>[4x]SNAMAKLRVGIVFGGKSAEHEVSLQSAKNIVDAIDKTRFDVVLLGIDKAGQWHVNDAENYLQNADDPAHIALRPSAISLAQVPGKHQHQLINAQNGQPLPTVDVIFPIVHGTLGEDGSLQGMLRVANLPFVGSDVLSSAACMDKDV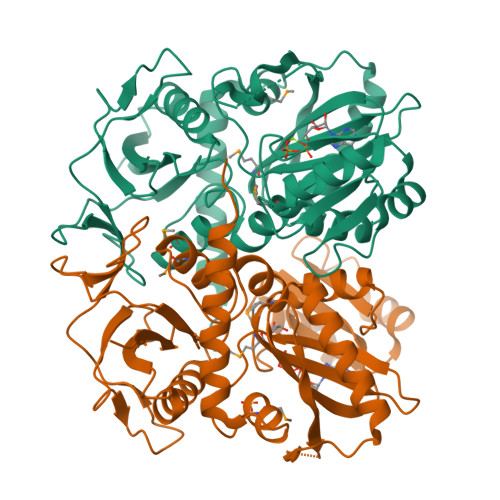AKRLLRDAGLNIAPFITLTRTNRHAFSFAEVESRLGLPLFVKPANQGSSVGVSKVANEAQYQQAVALAFEFDHKVVVEQGIKGREIECAVLGNDNPQASTCGEIVLNSEFYAYDTKYIDDNGAQVVVPAQIPSEVNDKIRAIAIQAYQTLGCAGMARVDVFLTADNEVVINEINTLPGFTNISMYPKLWQASGLGYTDLISRLIELALERHTANNALKTTM> MPLLLLLPLLWAGALAMDKLEFQICPKRCVCQILSPNLATLCAKKGLLFVPPNIDRRTVELRLADNFVTNIKRKDFANMTSLVDLTLSRNTISFITPHAFADLRNLRALHLNSNRLTKITNDMFSGLSNLHHLILNNNQLTLISSTAFDDVFALEELDLSYNNLETIPWDAVEKMVSLHTLSLDHNMIDNIPKGTFSHLHKMTRLDVTSNKLQKLPPDPLFQRAQVLATSGIISPSTFALSFGGNPLHCNCELLWLRRLSREDDLETCASPAL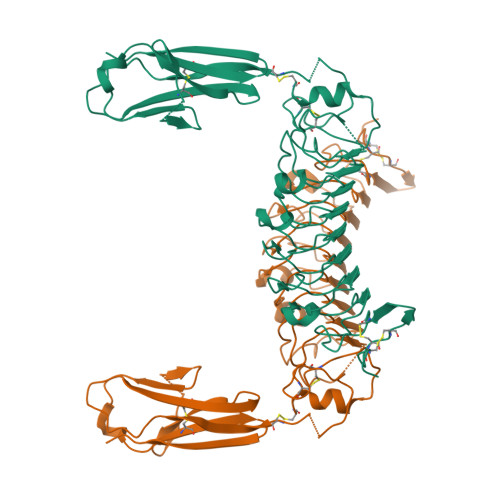LTGRYFWSIPEEEFLCEPPLITRHTHEMRVLEGQRATLRCKARGDPEPAIHWISPEGKLISNATRSLVYDNGTLDILITTVKDTGAFTCIASNPAGEATQTVDLHIIKGSEVLFQ>MAKVLCVLYDDPVDGYPKTYARDDLPKIDHYPGGQTLPTPKAIDFTPGQLLGSVSGELGLRKYLESNGHTLVVTSDKDGPDSVFERELVDADVVISQPFWPAYLTPERIAKAKNLKLALTAGIGSDHVDLQSAIDRNVTVAEVTYCNSISVAEHVVMMILSLVRNYLPSHEWARKGGWNIADCVSHAYDLEAMHVGTIAAGRIGLAVLRRLAPFDVHLHYTDRHRLPESVEKELNLTWHATREDMYPVCDVVTLNIPLHSPTEHMINDETLKLFKRGAYIVNTARGKLCDRDAVARALESGRLAGYAGDVWFP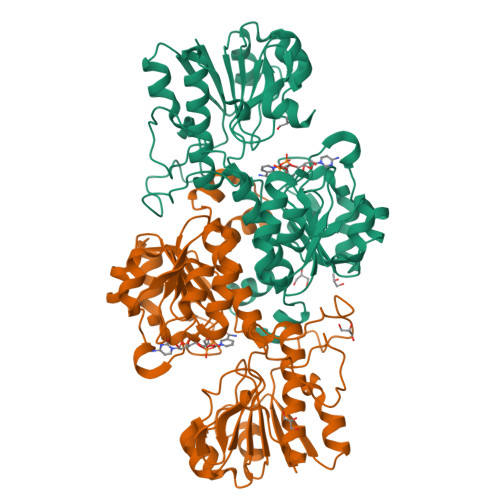QPAPKDHPWRTMPYNGMTPHISGTTLTAQARYAAGTREILECFFEGRPIRDEYLIVQGGALAGTGAHNYFKGNATGGSEEAAKFKKAV[2x]> MHHHHHHGSSKLKKLSEDSLTKQPEEVFDVLEKLGEGSYGSVFKAIHKESGQVVAIKQVPVESDLQEIIKEISIMQQCDSPYVVKYYGSYFKNTDLWIVMEYCGAGSVSDIIRLRNKTLIEDEIATILKSTLKGLEYLHFMRKIHRNIKAGNILLNTEGHAKLADFGVAGQLT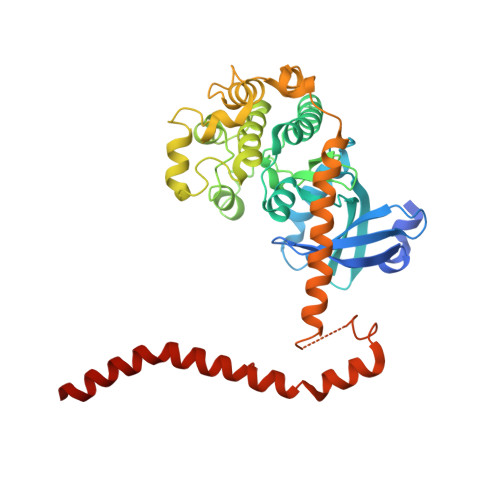DTMAKRNTVIGTPFWMAPEVIQEIGYNCVADIWSLGITSIEMAEGKPPYADIHPMRAIFMIPTNPPPTFRKPELWSDDFTDFVKKCLVKNPEQRATATQLLQHPFIKNAKPVSILRDLITEAMEIKAKRHEEQQRELEEEENWKVPQDGDFDFLKNLSLEELQMRLKALDPMMEREIEELRQRYTAKRQPILDAMDAKKRRQQNF> TYFITMNNARNFFIQQLESNAQDTATSLGLSLSQSLINHD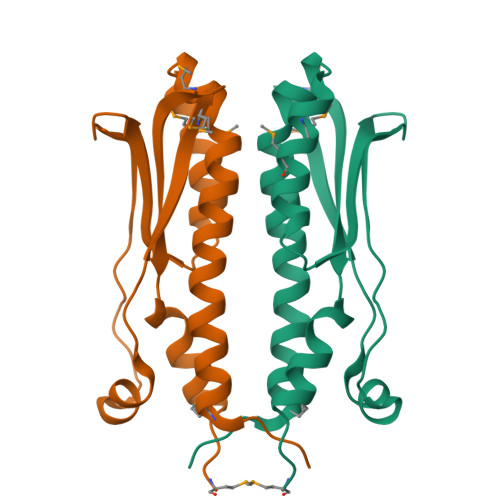VPTMDSMVKAVFDRGYFSSIKVQDIKGKVIILKKQLPQESDIPQWFVNLIKWPSTEKSSLIMDGWMQAGVVLVASDPSYVYASLWRNAVEM>[2x]SELRDRQAIFETLVAKGRELLACDRVIVYAFDDNYVGTVVAESVAEGWPQARDQVIEDPCFREHWVEAYRQGRIQATTDIFKAGLTECHLNQLRPLKVRANLVVPMVIDDQLFGLLIAHQASEPRQWQEIEIDQFSELASTGSLVLERLH

Of interest was PixJ from the thermophilic cyanobacterium Thermosynechococcus elongatus (Te), which transitions almost completely between blue light-absorbing Pb and green light-absorbing Pg end states using a phycoviolobilin (PVB) chromophore. In addition to the conventional thioether linkage that connects C522 within the GAF domain to the C31 carbon of the A pyrrole ethylidene side chain, PVB is attached via a second thioether linkage between C494 of the GAF domain and the C10 carbon between the B and C pyrrole rings. The end result is conversion of C10 from sp2 to sp3 hybridization, which shortens the π-conjugation system of PVB and induces the substantial hypsochromic shift from green- to blue-light absorption. Comparisons implied that photoconversion involves isomerization at the C15=C16 bond, a rupture of the C494–C10 thioether linkage, restoration of the π-conjugation between the B and C pyrrole rings, rotation and translation of the bilin in the GAF pocket, and conformational rearrangements of the protein backbone and surrounding amino acid side chains.

In our experiment, the temperature of a cryopreserved crystal was raised from 100 to 150 K, and a complete X-ray diffraction dataset of dark-adapted Pb was collected. As prior data with other CBCRs demonstrated that full photoconversion requires temperatures above 200 K, we anticipated that the blue light would generate one or more primary photoproducts and not drive rupture of the C494–C10 thioether linkage nor the complete transition to Pg. Indeed, comparisons of diffraction datasets collected at 150 K from a single TePixJ(GAF) crystal as Pb and then after irradiation with intense blue light clearly manifested structural changes at and around the chromophore. Isomorphous difference map peaks were highly localized to the D pyrrole ring for both units A and B. In fact, Fo(illuminated) − Fo(dark) maps around the D ring and the N535 side chain indicated electron density differences in excess of ±10 rmsd, which were consistent with structural changes in the bonds associated with C15 as PVB transitions toward Pg. Taken together, it appears that blue-light excitation at 150 K allowed isomerization of the chromophore within its binding pocket at the C15 methine bridge, and relaxation of N535 into a new orientation. Interestingly, the Fo − Fo difference peaks implied that PVB swings deeply into the binding pocket during the initial stages of photoconversion as compared with prior Pb and Pg models. The electron density differences revealed that PVB moves away from N535 after illumination, and now is in a better position to interact with the D492 and Q526 side chains, which move slightly to accommodate the new chromophore position. The binding-pocket side chains on helix α4 also adjusted slightly to the photoproduct, based on small difference peaks at Q526, H523, and C522.> MGSSHHHHHHSSGLVPRGSSEDFIETNPSGTNLESNYYKNETEAYAGLVAVYDVMRKYSGGFENTVSFLNAGSDDHVAGGGSSSDGAGIQGFSNFTINPTIMPRSYWSDFYQGIFRANVLLTKLPDVPMDESQIMRFTAETKALRALYYFNLVNMFRNVPLITEPLEPSEFNSVLQADPSAVYTQIEQDLNEAIGNLPDIISDDQKGRFSNGSAKALLGKVYLYQGKNQQAAAVLQEVNGTPGQTSQYGYKLLDNYDELWTVSNKFNSESILEVAHTNASGSGWGNWGQGTD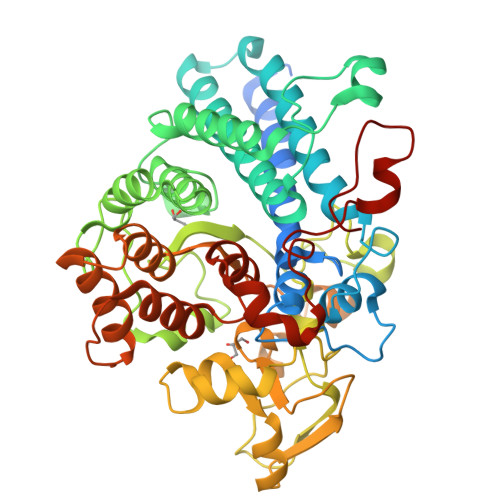EGNSINVMLGPRSYNQITEEAPDLPSGWSFNPVLPELYDLLEGDPRFEATILDLKALEEAGAASYVPGYQDTGYFLNKFIPRVTDVTTLTGEPVLNYRQNTYVIRLADTYLMEAEALGGSGARAQALLDAVRARVGLPSTPVSLTAIAKERRLELAGEGHRFYDLVRTGKAAEALSDRGFKAGVNEILPIPFQELQSTQIVQNPGY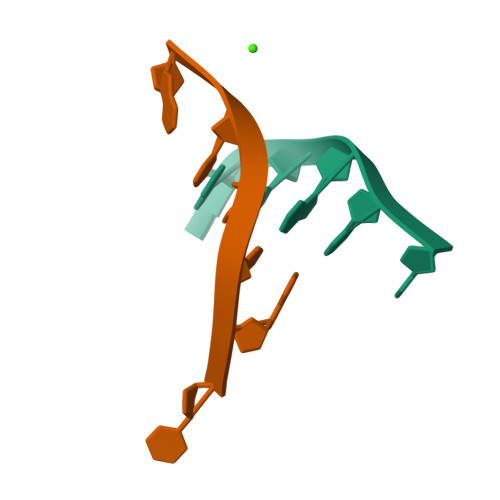>CGTACG[4x]> MAVKSIKVKLRLDDMPEIRAGLWKLHKEVNAGVRYYTEWLSLLRQENLYRRSPNGDGEQECDKTAEECKAELLERLRARQVENGHRGPAGSDDELLQLARQLYELLVPQAIGAKGDAQQIARKFLSPLADKDAVGGLGIAKAGNKPRWVRMREAGEPGWEEEKEKAETRKSADRTADVLRALADFGLKPLMRVYTDSEMSSVEWKPLRKGQAVRTWDRDMFQQAIERMMSWESWNQRVGQEYAKLVEQKNRFEQKNFVGQEHLVHLVNQLQQDMKEASPGLESKEQTAHYVTGRALRGSDKVFEKWGKLAPDAPFDLYDAEIKNVQRRNTRRFGSHDLFAKLAEPEYQALWREDASFLTRYAVYNSILRKLNHAKMFATFTLPDATAHPIWTRFDKLGGNLHQYTFLFNEFGERRHAIRFHKLLKVENGVAREVDDVTVPISMSEQLDNLLPRDPNEPIALYFRDYGAEQHFTGEFGGAKIQCRRDQLAHMHRRRGARDVYLNVSVRVQSQSEARGERRPPYAAVFRLVGDNHRAFVHFDKLSDYLAEHPDDGKLGSEGLLSGLRVMSVDLGLRTSASISVFRVARKDELKPNSKGRVPFFFPIKGNDNLVAVHERSQLLKLPGETESKDLRAIREERQRTLRQLRTQLAYLRLLVRCGSEDVGRRERSWAKLIEQPVDAANHMTPDWREAFENELQKLKSLHGICSDKEWMDAVYESVRRVWRHMGKQVRDWRKDVRSGERPKIRGYAKDVVGGNSIEQIEYLERQYKFLKSWSFFGKVSGQVIRAEKGSRFAITLREHIDHAKEDRLKKLADRIIMEALGYVYALDERGKGKWVAKYPPCQLILLEELSEYQFNNDRPPSENNQLMQWSHRGVFQELINQAQVHDLLVGTMYAAFSSRFDARTGAPGIRCRRVPARCTQEHNPEPFPWWLNKFVVEHTLDACPLRADDLIPTGEGEIFVSPFSAEEGDFHQIHADLNAAQNLQQRLWSDFDISQIRLRCDWGEVDGELVLIPRLTGKRTADSYSNKVFYTNTGVTYYERERGKKRRKVFAQEKLSEEEAELLVEADEAREKSVVLMRDPSGIINRGNW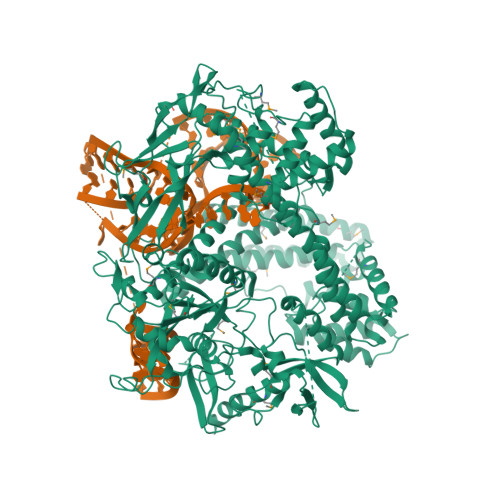TRQKEFWSMVNQRIEGYLVKQIRSRVPLQDSACENTGDILEHHHHHH>GSHMVERISLEKAALEFSEANAPHPRIYELPVEEGRSLLNEVQDSPVVKEDVDIEDIAVDTGEWGEINVRFIRPLHQEKKLPVIFYIHGAGWVFGNAHTHDKLIRELAVRTNSVVVFSEYSLSPEAKYPTAIEQNYAVLQQLKDFANDKKFDVNHLTVAGDSVGGNMATVMTLLTKQRGGQKIGQQVLYYPVTDANFDTDSYNEFAENYALTKEGMIWFWDQYTTSQEERHQITASPLRATKEDLADLPAALIITGEADVLRDEGEAYARKLREADVEVTQVRFQAIIHDFVMVNSMNETHATRAAMSLSTQWINEKNRK[8x]

In this study, we performed an in-depth biochemical and structural characterization of a novel microbial acetylesterase, LgEstI, from the bacterial fish pathogen Lactococcus garvieae. LgEstI belongs to the HSL family of α/β-hydrolases and presents a clear substrate preference for a short acyl chain and an acetate moiety that are suitable for the narrow entrance to the active site. Monomeric LgEstI exhibits a canonical α/β hydrolase fold with conserved key active site residues. The active site of LgEstI has the typical catalytic triad of esterases, identified as Ser159, Asp256, and His286, and is located at the bottom of the substrate access channel.

However, F207A exhibited a significantly increased hydrolytic activity (over 150%) toward pNA. To understand the increased activity of F207A against pNA at the molecular level, its structure was determined at a resolution of 2.1 Å. The overall structure of F207A was almost identical to that of wild-type LgEstI, with 0.177 of RMSD (Cα of monomer); in addition, the oligomerization form remained unchanged. No substantial movement around the active site was observed, implying that there could be multiple interactions among the residues that secure the interior conformation. However, Phe14 was shifted by approximately 0.5 Å due to the spatial reduction caused by the mutation of Phe207 to alanine. Phe14 in the wild-type protein interacted with Phe207 via edge-face interactions and was oriented toward the substrate access channel. The additional space created by the disappearance of Phe207 was partially occupied by Phe14. The pocket volume based on the molecular surface (MS) volume increased from 548.4 Å3 to 657.8 Å3 in the F207A structure. Therefore, area expansion could increase substrate accessibility and/or dissociation of the product, thereby increasing enzyme activity. The F207 mutation increased activity against pNA; however, F207A did not exhibit increased activity against other substrates with long acyl chains in parallel, when compared to LgEstI, indicating that other factors could be involved in substrate selectivity.>SNAMQEILSQLNKEIEGLKKAGLYKSERIITSPQNAEIKVGEKEVLNFCANNYLGLADHPALIKTAQTVVEQYGFGMASVRFICGTQTIHKELEKDISEFLGTDDTILYSSCFDANGGLFETLLGPEDAIISDELNHASIIDGIRLCKAQRYRYKNNAMGDLEAKLKEADEKGARFKLIATDGVFSMDGIIADLKSICDLADKYNALVMVDDSHAVGFIGENGRGTPEYCGVADRVDILTGTLGKALGGASGGYTSGHKEIIEWLRNRSRPYLFSNTVAPVIVATSLKVLELLKTEGPQLRKQLQENSRYFRAGMEKLGFQLVPGNHPIIPVMLGDAQLATNMADHLLQ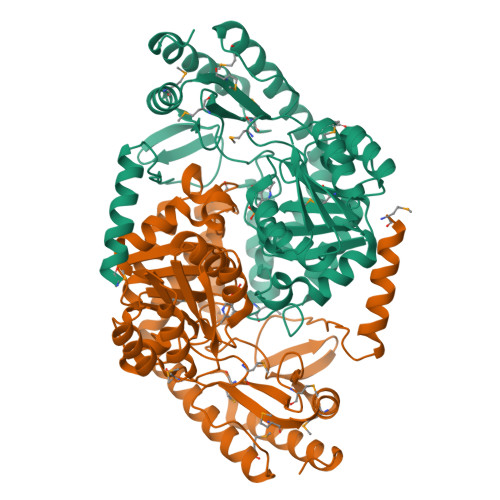EGIYVVGFSYPVVPMGKARIRVQMSAVHTQQQLDRAIEAFGQVGKKLGAI[2x]> GSSGSSGKDNIRHGVCWIYYPDGGSLVGEVNEDGEMTGE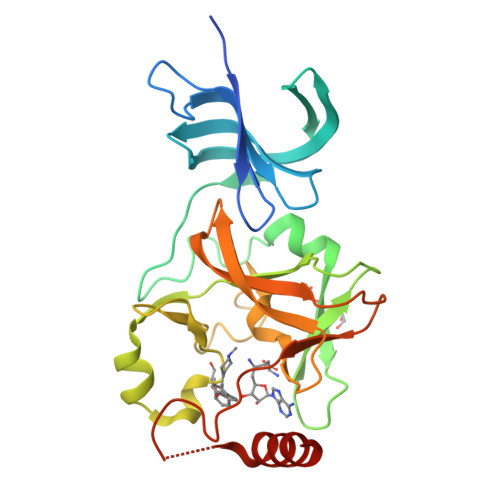KIAYVYPDERTALYGKFIDGEMIEGKLATLMSTEEGRPHFELMPGNSVYHFDKSTSSCISTNALLPDPYESERVYVAESLISSAGEGLFSKVAVGPNTVMSFYNGVRITHQEVDSRDWALNGNTLSLDEETVIDVPEPYNHVSKYCASLGHKANHSFTPNCIYDMFVHPRFGPIKCIRTLRAVEADEELTVAYGYDHSPPGKSGPEAPEWYQVELKAFQATQQK Here, we explore the viability of such a mechanism by inserting one de novo designed alpha beta protein into another such that the two beta sheets are combined into one. The backbone geometry at the junctions between the original domains is regularized, and the sequence at the newly formed interface is optimized to stabilize the single integrated domain structure. Crystal structures of two such proteins demonstrate that complex beta sheet structures can be designed with considerable accuracy using this approach and provide a proof-of-concept for the hypothesis that complex beta topologies in natural proteins may have evolved from simpler beta sheet structures in a similar manner. Our success in designing larger beta sheet domains by recombining smaller independently folded beta sheet proteins suggests a similar mechanism could have played a role in the evolution of naturally occurring complex beta sheet proteins.

A second extended sheet protein was created by inserting one designed ferredoxin domain into another to create a half-barrel structure with four alpha helices and six beta strands. A beta turn segment between two beta strands of the host ferredoxin was removed and the resulting cut-points in the host beta strands were linked to two beta strand cut-points in the insert, fusing the two strand pairs into a single, longer pair at the center of a six-stranded beta sheet. CD spectra show that the protein contains both alpha and beta structures. Crystals were obtained which diffracted to 3.3Å resolution. Attempts to improve these statistics by rebuilding portions of the model proved unsuccessful, possibly due to a register shift or dynamic fluctuations in the structure (perhaps corresponding to slightly 'molten-globule'-like behavior) that are difficult to computationally model. However, unbiased low-resolution omit maps suggest that the overall topology is correct. In the model that displays the best refinement statistics, the protein backbone was similar to the design model with a C-alpha RMSD value of 2 Å. The fused beta sheet aligns with the design model, while the inter-domain helices shift slightly to accommodate the inter-domain interface. The most similar SCOP domains had weak TM-align scores (0.54 and 0.51), and the sheets in these matched structures have different connectivities than those of the designs, suggesting that the two designed proteins have novel folds.

> MEMDIRFRGDDPEAYYKALREMIRQARKFAGTVTVTLIIRFRGDDLEALEKALKEMIRQARKFAGTVTYTLDGNDLEIRITGVPPQVILELVKEAIRLAKEFNITVTVELVIRITGVPEQVRKELAKEAERLAKEFNITVTYTIRL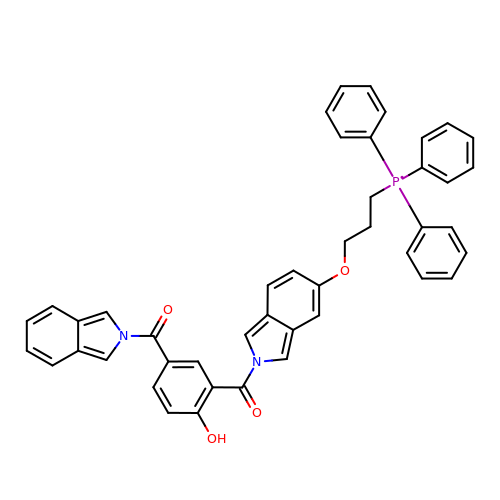[2-hydroxy-5-(2H-isoindole-2-carbonyl)phenyl]{5-[3-(triphenyl-lambda~5~-phosphanyl)propoxy]-2H-isoindol-2-yl}methanone | C45 H37 N2 O4 P | LKRQAENWLOVTOO-UHFFFAOYSA-N> ELSENFKKLMKYPYRPCTCTRCIEEQRVSAWFDERFNRSMQPLLTAKNAHLEEDTYKWWLRLQREKQPNNLNDTIRELFQVVPGNVDPLLEKRLVSCRRCAVVGNSGNLKESYYGPQI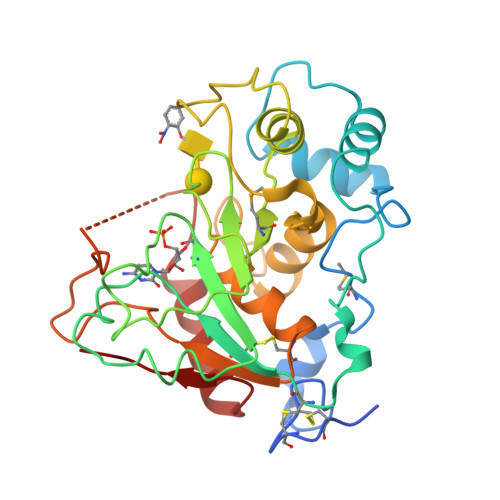DSHDFVLRMNKAPTEGFEADVGSKTTHHFVYPESFRELAQEVSMILVPFKTTDLEWVISATTTGRISHTYVPVPAKIKVKKEKILIYHPAFIKYVFDRWLQGHGRYPSTGILSVIFSLHICDEVDLYGFGADSKGNWHHYWENNPSAGAFRKTGVHDGDFESNVTTILASINKIRIFKGR>[2x]SNAMNKTLIINAHPKVDDTSSVSIKVFKHFLESYKELISNNETIEQINLYDDVVPMIDKTVLSAWEKQGNGQELTREEQ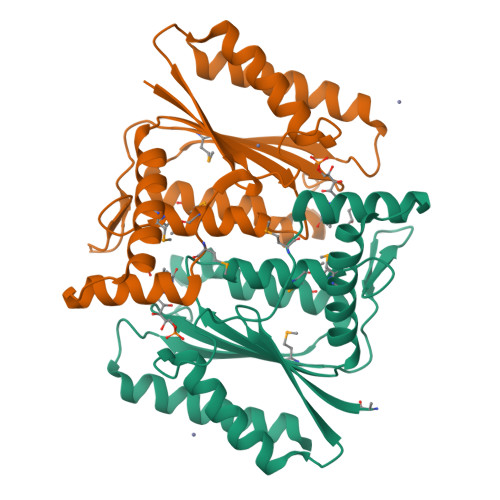KVTERMSEILQQFKSANTYVIVLPLHNFNIPSKLKDYMDNIMIARETFKYTETGSVGLLKDGRRMLVIQASGGIYTNDDWYTDVEYSHKYLKAMFNFLGIEDYQIVRAQGTAVLDPTEVLQNAYKEVEEAASRLANKYIFSLEE> MTAKDDYPSLSFQQDYVYIFSSDFQLSEELGVALINALSAKEIVPERLYVMLNDKTISFSF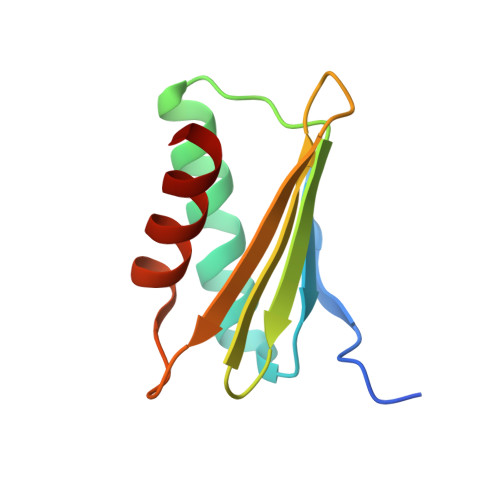ISKNKKSKNRVLSTEKKLNYKHISEYIVNEIEY> GAMGMGLAGGSLPSLAPDLVRDLIATAADISLLVSQEGVVREVMANPHHPSFGQLSEWEGRPLEEVLTAESVAKFRLRSEGLEPGRGSVAVELNHIDPRSFEFPIRYILHRLPADRSILMLGRDLRPIAEVQQQLVAAQLAMERDYETQREMETRYRVVLDVSRDPMVLVSMSTGRIVDLNSAAGLLLGGVRQDLLGAAIAQEFEGR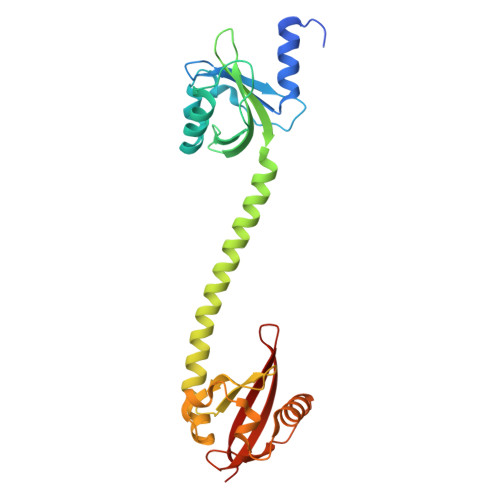RRGEFMETMTNLAATESAAPVEVLARRSQKRLLVVPRVFRAAGERLLLCQIDPAD> TYSNLG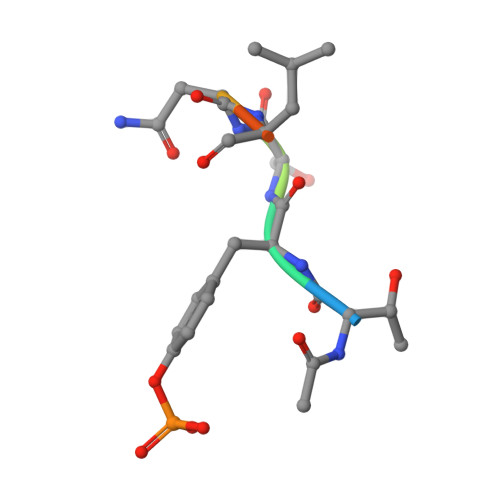Q>[4x]EDNSLSQKKKVTVEDLFSEDFKIHDPEAKWISDTEFIYREQKGTVRLWNVETNTSTVLIEGKKIESLRAIRYEISPDREYALFSYNVEPIYQHSYTGYYVLSKIPHGDPQSLDPPEVSNAKLQYAGWGPKGQQLIFIFENNIYYCAHVGKQAIRVVSTGKEGVIYNGLSDWLYEEEILKTHIAHWWSPDGTRLAYAAINDSRVPIMELPTYTGSIYPTVKPYHYPKAGSENPSISLHVIGLNGPTHDLEMMPPDDPRMREYYITMVKWATSTKVAVTWLNRAQNVSILTLCDATTGVCTKKHEDESEAWLHRQNEEPVFSKDGRKFFFIRAIPQGGRGKFYHITVSSSQPNSSNDNIQSITSGDWDVTKILAYDEKGNKIYFLSTEDLPRRRQLYSANTVGNFNRQCLSCDLVENCTYFSASFSHSMDFFLLKC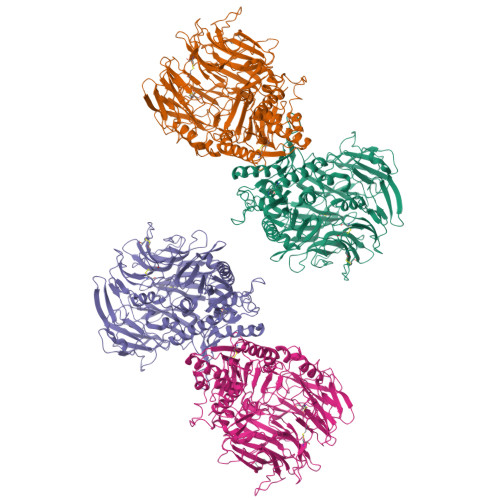EGPGVPMVTVHNTTDKKKMFDLETNEHVKKAINDRQMPKVEYRDIEIDDYNLPMQILKPATFTDTTHYPLLLVVDGTPGSQSVAEKFEVSWETVMVSSHGAVVVKCDGRGSGFQGTKLLHEVRRRLGLLEEKDQMEAVRTMLKEQYIDRTRVAVFGKDYGGYLSTYILPAKGENQGQTFTCGSALSPITDFKLYASAFSERYLGLHGLDNRAYEMTKVAHRVSALEEQQFLIIHPTADEKIHFQHTAELITQLIRGKANYSLQIYPDESHYFTSSSLKQHLYRSIINFFVECFRI> GAGCAGACCAGA;> CGGGACTCA;> TCTCCG;> TCTGAGTCGGTCTGC

In this work, we exhaustively probe the ability of all 36 immobile HJ sequences to form DNA crystals in two different designed systems. Three separate self-assembling DNA crystal systems are described in this report: the “4 × 5” and “4 × 6” designs (collectively referred to as the 4 × N systems), and a third construct with a “scrambled” sequence variant of the 4 × 6 lattices. Self-assembly was mediated by three constituent oligonucleotides: (S1) containing four sequence repeats of either 5 or 6 bases; (S2) composed of 21 bases containing complementary regions to both (S1); and (S3) which forms the second junction crossover. The HJ serves as the fundamental component at the core of each unit, and the ultimate assembly of the full lattice is facilitated by the complementary 2-base sticky ends that tail each duplex.

Seventeen of the 36 junctions successfully crystallized, a 47% success rate. Because the 4 × 6 system yielded R3 symmetry in 5 of 17 junctions, we considered whether the downstream sequences adjacent to the junction could play a role in crystallization efficiency, junction angle, and symmetry preference, or if the HJ alone was the singular determinant. In crystals containing R3 symmetry, the average cell for each was a = b = 114.9 Å c = 49.77 Å with the c-axis confined to a tighter regime (σ = 0.75). The cavity volumes were also markedly different from the P32 cavity volumes (~614.7  nm3) compared with ~532.1 nm3 in the more densely packed R3 structure (see Supplementary Fig. 11 for calculation details). The average junction angles of 54.60° (σ = 1.44) and 58.37° (σ = 2.3) for the P32 and R3 symmetries, respectively, along with their preference for salts or organic solvents, were likely the major contributing factors that yielded the divergent lattices. However, in the majority of the crystal structures reported here, the cacodylate anion indeed fits best into the electron density map of our X-ray structures, due to the presence of sodium cacodylate in the crystallization solution.Pentameric ligand-gated ion channels (pLGICs) mediate synaptic transmission and are sensitive to their lipid environment. We demonstrate that the model pLGIC, ELIC (Erwinia ligand-gated ion channel), is positively modulated by the anionic phospholipid, phosphatidylglycerol, from the outer leaflet of the membrane. To investigate the mechanism of positive modulation by POPG, we determined structures of WT ELIC by single particle cryo-electron microscopy (cryo-EM) in the absence and presence of agonist in MSP1E3D1 nanodiscs with 2:1:1 POPC:POPE:POPG (hereafter referred to as 2:1:1) or POPC. In combination with streamlined alchemical free energy perturbation calculations and functional measurements in asymmetric liposomes, the data support a mechanism by which an anionic phospholipid stabilizes the activated, open-channel state of a pLGIC by specific, state-dependent binding to this site.

We began with the previously reported gain-of-function triple mutant V261Y/G319F/I320F (ELIC3)33 that introduces three aromatic residues at the top of the M4 helix (M4). As previously reported, ELIC3 caused a left-shift in the agonist dose response curve, slowed desensitization in the presence of agonist, and slowed deactivation as assessed by excised patch-clamp recordings from 2:1:1 giant liposomes. Interestingly, the structure of agonist-bound ELIC3 in 2:1:1 nanodiscs, determined at 3.3 Å resolution, showed opening of the pore at 16′ but still occlusion at 9′. The ELIC3 gain-of-function mutant further opens at 16′ with the F247 side chain turning away from the pore into an intersubunit space, but otherwise resembles the WT structure. The patch-clamp and Tl+ flux data of WT and ELIC3 show robust activation and desensitization in 2:1:1 membranes such that agonist-bound structures of WT and ELIC3 are expected to show desensitized conformations. However, the observed structures are most consistent with pre-active conformations based on structures of other pLGICs, especially the nAchR, where 16′ and 9′ appear to be activation gates and desensitization consistently involves a constriction in the most intracellular aspect of the pore. Therefore, we cannot confidently assign the WT and ELIC3 agonist-bound structures as pre-active or desensitized conformations, and further work is necessary to clarify their annotation.

>[5x]APADNAADARPVDVSVSIFINKIYGVNTLEQTYKVDGYIVAQWTGKPRKTPGDKPLIVENTQIERWINNGLWVPALEFINVVGSPDTGNKRLMLFPDGRVIYNARFLGSFSNDMDFRLFPFDRQQFVLELEPFSYNNQQLRFSDIQVYTENIDNEEIDEWWIRGKASTHISDIRYDHLSSVQPNQNEFSRITVRIDAVRNPSYYLWSFILPLGLIIAASWSVFWLESFSERLQTSFTLMLTVVAYAFYTSNILPRLPYTTYIDQMIIAGYGSIFAAILLIIFAHHRQANGVEDDLLIQRCRLAFPLGFLAIGCVLVIRFFTL>MSMEPTLQSILDQRSLRWIFVGGKGGVGKTTTSCSLAIQ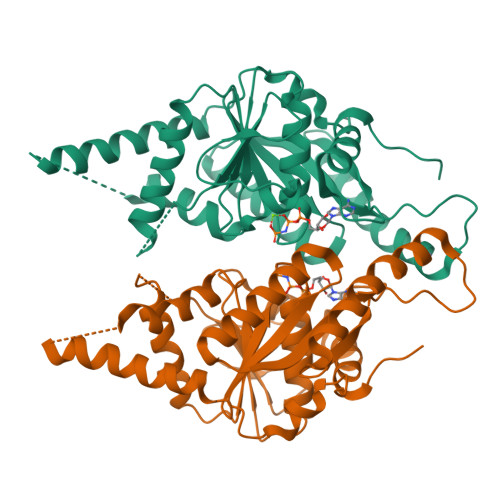LAKVRRSVLLLSTDPAHNLSDAFSQKFGKEARLVEGFDNLYAMEIDPNGSMQDLLAGQTGDGDAGMGGVGVMQDLAYAIPGIDEAMSFAEVLKQVNSLSYETIVFDTAPTGHTLRFLQFPTVLEKALAKVSQLSGQYGSLLNGILGGSGTLPNGQTLSDVMEKLDSLRVTISEVNAQFKDERLTTFVCVCIPEFLSLYETERMIQELANYGIDTHCIVVNQLLFPKPGSDCEQCTARRRMQKKYLDQIEELYDEEFNVVKMPLLVEEVRGKERLEKFSEMLIKPFVPPEHHHHHH[2x]3-FLUOROBENZENE-1,2-DIOL | C6 H5 F 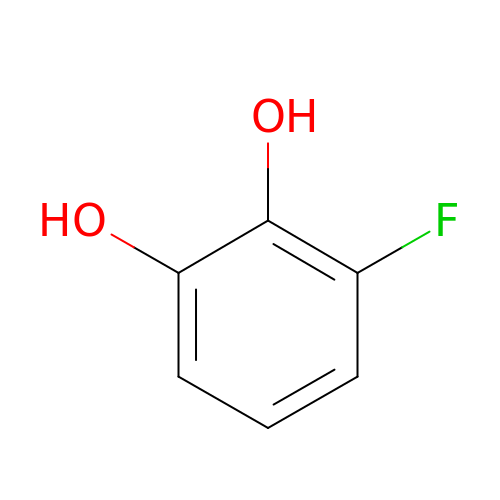O2 | DXOSJQLIRGXWCF-UHFFFAOYSA-N>[2x]MPNIKIFSGSSHQDLSQKIADRLGLELGKVVTKKFSNQETCVEIGESVRGEDVYIVQSGCGEINDNLMELLIMINACKIASASRVTAVIPCFPYARQDKKDKSRAPISAKLVANMLSVAGADHIITMDLHASQIQGFFDIPVDNLYAEPAVLKWIRENISEWRNCTIVSPDAGGAKRVTSIADRLNVDFALIHKERKKANEVDRMVLVGDVKDRVAILVDDMADTCGTICHAADKLLSAGATRVYAILTHGIFSGPAISRINNACFEAVVVTNTIPQEDKMKHCSKIQVIDISMILAEAIRRTHNGESVSYLFSHVPLLEHHHHHH

PRPP is formed from ATP and D-ribose-5-phosphate (R5P) by the phosphoribosyl pyrophosphate synthetases (PRSs). The human PRS family, which has 3 isoforms (hPRS1, hPRS2 and hPRS3), belongs to the class I PRSs that requires divalent metal ions such as Mg2+ as the activator, inorganic phosphate ion for activity, and ATP or dATP as the diphosphoryl donor. Due to the important role of PRPP in the nucleotide metabolic process, the stability of PRPP content is essential for cell physiology and is predominantly controlled by hPRS1, the ubiquitously expressed human PRPP synthetase. Mutations in hPRS1 affect vital cell functions and are related to many diseases and disorders.

2− complex was determined using the MR method to 2.0 Å resolution. More information about the 2.0 Å resolution structure could be found in the supplementary materials (S1). 2− complex structure, the β9–10 strands from Arg196 to Val202, with missing electron density, are possibly structurally and functionally similar to the same region in the Thermoplasma volcanium PRS-R5P complex. We also found that the highly conserved residues Lys194 and Arg196 (located between the β9–10 strands) exist among all 3 classes of PRS. The second motif with conformational change, termed as the flexible loop (from Ile89 to Ile107), exists among all known PRS structures. According to the crystallography symmetry operation, the PRS1 crystal structure appeared as a three-leaf clover like hexahydric ring that matched the apo state of the PRS1 3D-EM structure. We then reconstructed the 3D- EM structure of the PRS1 apo form, which displays the 3-leaf clover structure that matches the PRS1 hexamer model derived from the crystal structure, according to the crystallography symmetry operation. Based on the EM results and the crystal structure, the functional hexamer might be the most efficient functional form. The surfaces of active centers and interfaces are highly conserved according to our surface conservation analysis.> MKIINSDQKVKITLKINGEKYETEVEPRRLLVHVLRELGFTGVHIGCDTSNCGACTVIMNGKSVKSCTVLAVEADGAEILTVEGLAKDGKLHPIQEAFWENHALQCGYCTPGMIMEAYWL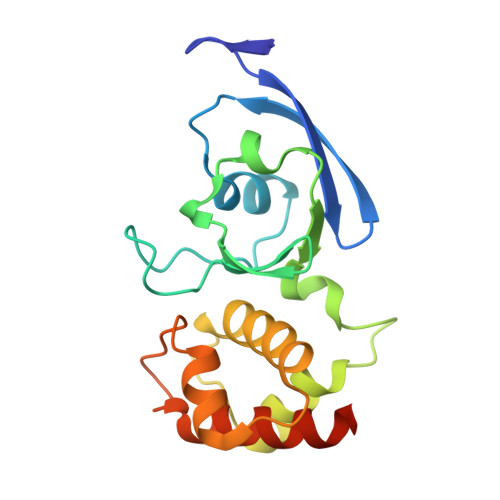LREKPNPTEEEIREGISGNLCRCTGYQNIVKAIKAAAEKLSQTPYQHQ> HKCDITLQAIIKTLNSLTEQKTLCTELTVTDIFAASKNTTEKETFCRAATV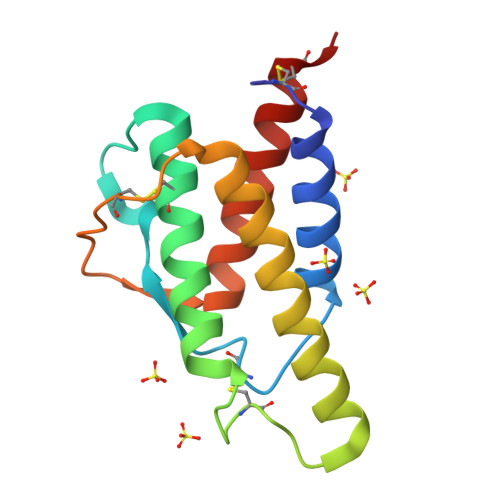LRQFYSHHEKDTRCLGATAQQFHRHKQLIRFLKRLDRNLWGLAGLNSCPVKEANQSTLENFLERLKTIMREKYSKCSS> GHDCHLSDMLQQLHSVNASKPSERGLVRQEEAEDPACIPIFWVSKWVDYSDKYGLGYQLCDNSVGVLFNDSTRLILYNDGDSLQYIERDGTESYLTVSSHPNSLMKKITLLKYFRNYMSEHLLKAGANITPREGDELARL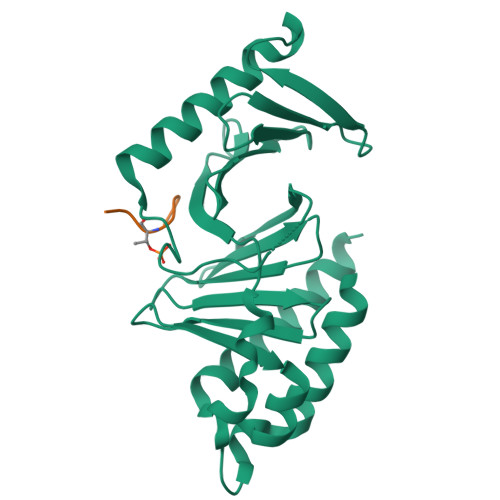PYLRTWFRTRSAIILHLSNGSVQINFFQDHTKLILCPLMAAVTYIDEKRDFRTYRLSLLEEYGCCKELASRLRYARTMVDKLLSSR;> PISSTPL> MVPISPIETVPVKLKPGMDGPKVKQWPLTEEKIKALVEICTEMEKEGKISKIGPENPYNTPVFAIKKKDSTKWRKLVDFRELNKRTQDFWEVQLGIPHPAGLKQKKSVTVLDVGDAYFSVPLDKDFRKYTAFTIPSINNETPGIRYQYNVLPMGWKGSPAIFQCSMTKILEPFRKQNPDIVIYQYMDDLYVGSDLEIGQHRTKIEELRQHLLRWGFTTPDKKHQKEPPFLWMGYELHPDKWTVQPIVLPEKDSWTVNDIQKLVGKLNWASQIYAGIKVRQLCKLLRGTKALTEVVPLTEEAELELAENREILKEPVHGVYYDPSKDLIAEIQKQGQGQWTYQIYQEPFKNLKTGKYARMKGAHTNDVKQLTEAVQKIATESIVIWGKTPKFKLPIQKETWEAWWTEYWQATWIPEWEFVNTPPLVKLWYQLEKEPIIGAETFYVDGAANRETKLGKAGYVTDRGRQKVVPLTDTTNQKTELQAIHLALQDSGLEVNIVTDSQYALGIIQAQPDKSESELVSQIIEQLIKKEKVYLAWVPAHKGIGGNEQVDKLVSAGIRKVL;> MGHHHHHHMVPISPIETVPVKLKPGMDGPKVKQWPLTEEKIKALVEICTEMEKEGKISKIGPENPYNTPVFAIKKKDSTKWRKLVDFRELNKRTQDFWEVQLGIPHPAGLKQKKSVTVLDVGDAYFSVPLDKDFRKYTAFTIPSINNETPGIRYQYNVLPQGWKGSPAIFQCSMTKILEPFRKQNPDIVIYQYMDDLYVGSDLEIGQHRTKIEELRQHLLRWGFITPDKKHQKEPPFLWMGYELHPDKWTVQPIVLPEKDSWTVNDIQKLVGKLNWASQIYAGIKVRQLCKLLRGTKALTEVVPLTEEAELELAENREILKEPVHGVYYDPSKDLIAEIQKQGQGQWTYQIYQEPFKNLKTGKYARMKGAHTNDVKQLTEAVQKIATESIVIWGKTPKFKLPIQKETWEAWWTEYWQATWIPEWEFVNTPPLVKLWYQ

Certain nucleotide reverse transcriptase (RT) inhibitors (NRTIs) such as tenofovir and lamivudine can inhibit both HBV Pol and Human immunodeficiency virus 1 (HIV-1) RT, leading to speculation on structural and mechanistic analogies between the deoxynucleotide triphosphate (dNTP)-binding sites of these enzymes. The Q151M mutation in HIV-1 RT, located at the dNTP-binding site, confers resistance to various NRTIs, while maintaining sensitivity to tenofovir and lamivudine. The residue corresponding to Gln151 is strictly conserved as a methionine in HBV Pol. Therefore, the structure of the dNTP-binding pocket of the HIV-1 RT Q151M mutant may reflect that of HBV Pol.

Here, the crystal structure of HIV-1 RT Q151M, determined at 2.6 Å resolution, in a new crystal form with space group P321 is presented. HIV-1 RT Q151M was crystallized in the trigonal space group P321, with one p66/p51 heterodimer in the asymmetric unit. Although the structure of HIV-1 RT Q151M superimposes well onto that of HIV-1 RT in a closed conformation, a slight movement of the β-strands (β2–β3) that partially create the dNTP-binding pocket was observed. This movement might be caused by the introduction of the bulky thioether group of Met151. Gln151 in motif B interacts directly with the 3′-OH of the incoming dNTP and the conserved Arg72 via hydrogen bonds. The structural analysis in this study also showed clear electron density for the Met151 residue, which indicated that the side chain of Met151 is flipped out from the dNTP-binding pocket and is exposed to the solvent. The structure also highlighted the possibility that the hydrogen-bonding network among amino acids and NRTIs is rearranged by the Q151M mutation, leading to a difference in the affinity of NRTIs for HIV-1 RT and HBV Pol. The structural comparison also suggests that hydrophobic interactions between the methyl group of TNV and the thioether group of methionine might compensate for the loss of hydrogen bonds; hence, tenofovir exhibits an inhibitory action towards both HIV-1 RT Q151M and HBV Pol.> SEGSDAPNFVLEDTNGKRIELSDLKGKGVFLNFWGTWCPHCKKEFPYMANQ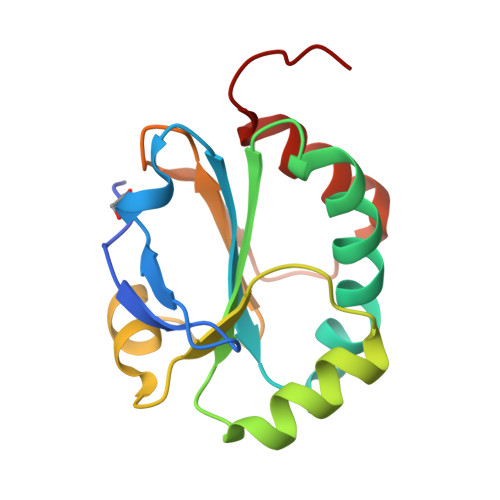YKHFKSQGVEIVAVNVGESKIAVHNFMKSYGVNFPVVLDTDRQVLDAYDVSPLPTTFLINPEGKVVKVVTGTMTESMIHDYMNLIKPGETSG3'-{4-[(4-amino-2-oxopyrimidin-1(2H)-yl)methyl]-1H-1,2,3-triazol-1-yl}-3'-deoxyadenosine 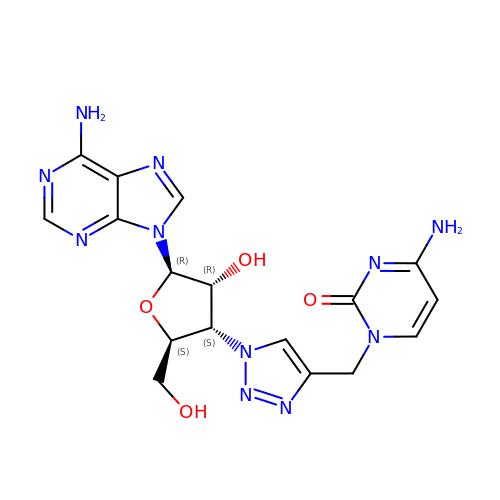| C17 H19 N11 O4 | RYUXRYKLIYXCJZ-RVXWVPLUSA-N> MPSSSSEDAQGGNRFECVSNSTSPRRKNATKDEAACLQP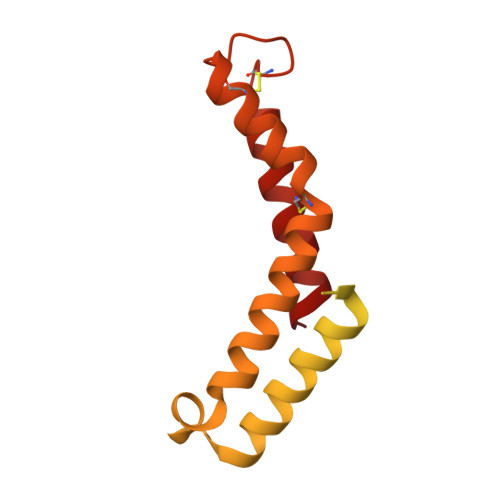RRSAVSGPREDVLCIRTTPQPHVRRGKSGPGRRKRMRFGRERERRDKKRGEGERKRTRFPFLRLHIEGGNANSRRPLCFPSRHSLLRNHYGSLSMAFRKVSPPKAPMSVFEARSSFLDLEQCARAAGPQRWEAECQGVRQRALQAAADVMSRECGAYGDSFFQCYRHGFRLEACQGEKATMQLLRCQRMVADRLVPL>MASTVSNTSKLEKPVSLIWGCELNEQNKTFEFKVEDDEEKCEHQLALRTVCLGDKAKDEFHIVEIVTQEEGAEKSVPIATLKPSILPMATMVGIELTPPVTFRLKAGSGPLYISGQHVA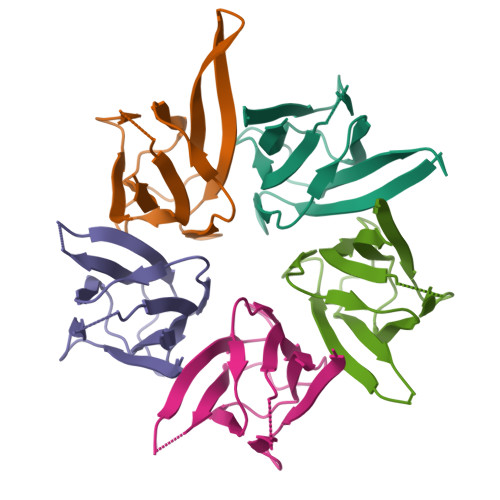MEEDY[5x]> MSTFKNEMNGNNLLHVAVLAFPFGTHAAPLLSLVKKIATEAPKVTFSFFCTTTTNDTLFSRSNEFLPNIKYYNVHDGLPKGYVSSGNPREPIFLFI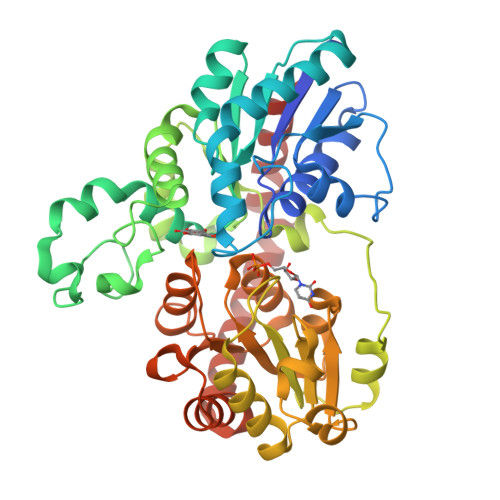KAMQENFKHVIDEAVAETGKNITCLVTDAFFWFGADLAEEMHAKWVPLWTAGPHSLLTHVYTDLIREKTGSKEVHDVKSIDVLPGFPELKASDLPEGVIKDIDVPFATMLHKMGLELPRANAVAINSFATIHPLIENELNSKFKLLLNVGPFNLTTPQRKVSDEHGCLEWLDQHENSSVVYISFGSVVTPPPHELTALAESLEECGFPFIWSFRGDPKEKLPKGFLERTKTKGKIVAWAPQVEILKHSSVGVFLTHSGWNSVLECIVGGVPMISRPFFGDQGLNTILTESVLEIGVGVDNGVLTKESIKKALELTMSSEKGGIMRQKIVKLKESAFKAVEQNGTSAMDFTTLIQIVTS>[4x]GMQTLNDIYLAYLDSL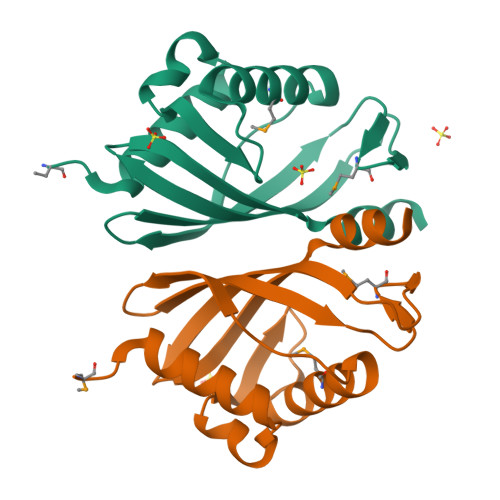NHQAFDELGTFVDDNVEHNGRPFGLSGYRDMLVKDFADIPDLRFEAEILVSDATRLAARLFFDCTPKSIFMDLPVNGRRVQFCEHVFYDFEQAKIRRVWSVLDKVAIERQLG> MAVKVEYDLKRLRNIVIAAHIDAGKTTTTERILYYTGRIHKIGEVHEGAATMDFMEQERERGITITAAVTTCFWKDHRINIIDTPGHVDFTIEVERSMRVLDGAIVVFDSSQGVEPQSETVWRQAEKYKVPRIAFANKMDKTGADLWLVIRTMQERLGARPVVMQLPIGREDTFSGIIDVLRMKAYTYGNDLGTDIREIPIPEEYLDQAREYHEKLVEVAADFDENIMLKYLEGEEPTEEELVAAIRKGTIDLKITPVFLGSALKNKGVQLLLDAVVDYLPSPLDIPPIKGTTPEGEVVEI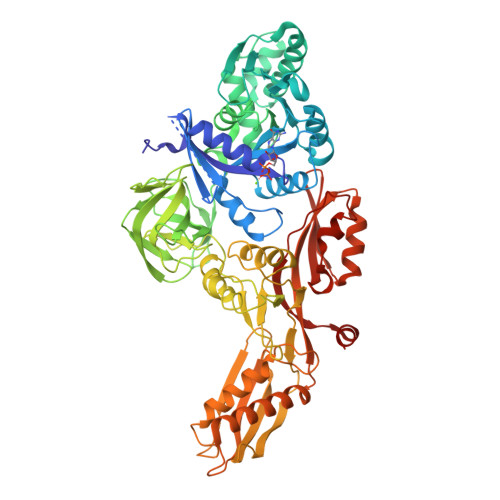HPDPNGPLAALAFKIMADPYVGRLTFIRVYSGTLTSGSYVYNTTKGRKERVARLLRMHANHREEVEELKAGDLGAVVGLKETITGDTLVGEDAPRVILESIEVPEPVIDVAIEPKTKADQEKLSQALARLAEEDPTFRVSTHPETGQTIISGMGELHLEIIVDRLKREFKVDANVGKPQVAYRETITKPVDVEGKFIRQTGGRGQYGHVKIKVEPLPRGSGFEFVNAIVGGVIPKEYIPAVQKGIEEAMQSGPLIGFPVVDIKVTLYDGSYHEVDSSEMAFKIAGSMAIKEAVQKGDPVILEPIMRVEVTTPEEYMGDVIGDLNARRGQILGMEPRGNAQVIRAFVPLAEMFGYATDLRSKTQGRGSFVMFFDHYQEVPKQVQEKLIKGQ>[12x]MIDLKQYEFWFLVGSQYLYGLETLKKVEQQASKIVDSLNDDPIFPSKIVLKPVLKSSSEITEIFEKANADPKCAGVIVWMHTFSPSKMWIRGLSINKKPLLHLHTQYNREIPWDTIDMDYMNLNQSAHGDREHGFIHARMRLPRKVVVGHWEEKEVREKIAKWMRVACA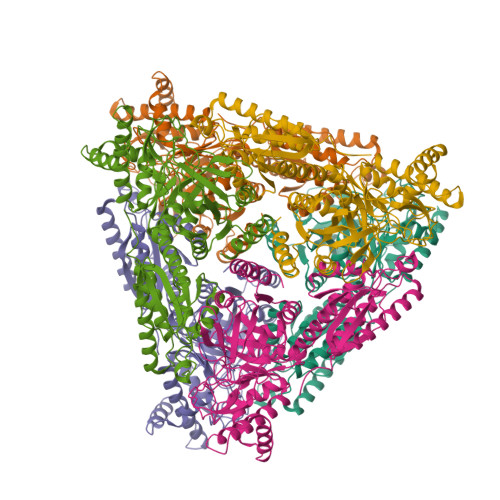IQDGRMGQIVRFGDNMREVASTEGDKVEAQIKLGWSINTWGVGELAERVKAVPEREVEELLKEYREKYIMPEDEYSLKAIREQAKIEIALREFLAAANAVGFTTTFEDLHDLPQLPGLAVQRLMEEGYGFGAEGDWKAAGLVRAIKVMGTSLPGGTSFMEDYTYHLTPGNELVLGAHMLEVCPTIAKEKPRIEVHPLSIGGKADPARLVFDGQEGPAVNASIVDMGNRFRLVVNKVLSVPIERKMPKLPTARVLWKPLPDFKRATTAWILAGGSHHTAFSTAIDVEYLIDWAEALEIEYVVIDENLDLEDFKKELRWNELYWGLLKR> MTKVDFWPTLKDA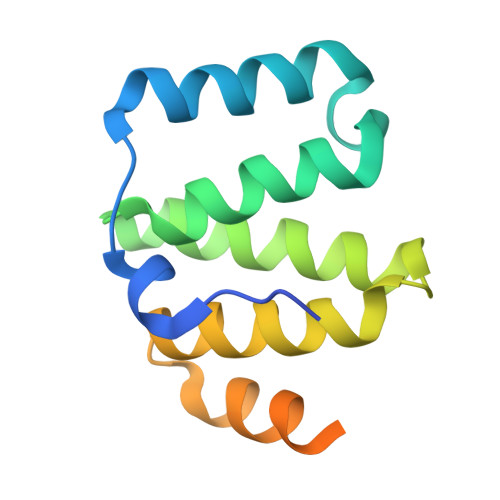YEPLYPQQLEILRQQVVSEGGPTATIQSRFNYAWGLIKSTDVNDERLGVKILTDIYKEAESRRRECLYYLTIGCYKLGEYSMAKRYVDTLFEHERNNKQVGALKSMVEDKIQKETL>GSHMDSTTIQQNKDTLSQIVVFPTGNYDKNEANAMVNRLANIDGKYLNALKQNNLKIKLLSGKLTDEKEYAYLKGVVPEGWEGTGKTWDDVPGLGGSTVALRIGFSNKGKGHDAINLELHETAHAIDHIVLNDISKSAQFKQIFAKEGRSLGNVNYLGVYPKEFFAES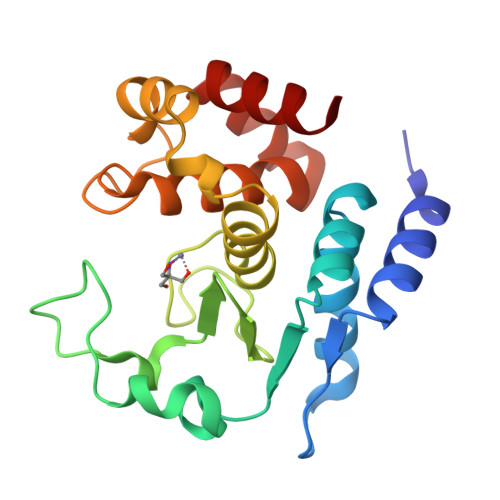FAYYYLNQDTNSKLKSACPQTYSFLQNLAK[2x]> MGRIKNKQFAVIGLGRFGGSIVKELHRMGHEVLAVDINEEKVNAYASYATHAVIANATEENELLSLGIRNFEYVIVAIGANIQASTLTTLLLKELDIPNIWVKAQNYYHHKVLEKIGADRIIHPEKDMGVKIAQSLSDENVLNYLEGS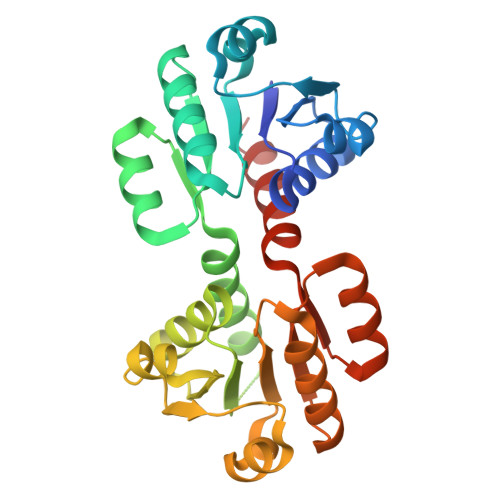KQFAVIGLGRFGGSIVKELHRMGHEVLAVDINEEKVNAYASYATHAVIANATEENELLSLGIRNFEYVIVAIGANIQASTLTTLLLKELDIPNIWVKAQNYYHHKVLEKIGADRIIHPEKDMGVKIAQSLSDENLELVPR The structural and zinc-binding properties of PA4063, one of the periplasmic proteins expressed by Pseudomonas aeruginosa under zinc-deficient conditions, are presented. PA4063 has a noncanonical ferredoxin-like fold. Two zinc-binding sites with micromolar affinity are exposed and are located on the same face of the structure. Two histidine-rich loops, which are disordered in the apoprotein, contribute to zinc coordination in one of the sites. These findings strongly suggest a role for PA4063 in zinc trafficking, possibly acting as a metal chaperone or as a regulator of a transport system.

PA4063 crystallized in two different forms corresponding to space groups P41212 and P65. The asymmetric unit of the hexagonal crystal comprises three protein molecules, but the interactions are so limited that they can be considered as simple packing contacts between monomers as in the case of the tetragonal crystal form. This observation is in line with size-exclusion chromatography, which shows that the protein is monomeric in solution regardless of the presence of zinc. Despite the differences in crystal packing with regard to both lattice and asymmetric unit composition, the conformation of the protein in the two crystal forms is almost identical (Cα r.m.s.d. in the range 0.49–0.74 Å).

>HDDHDHDHAHGSLGKHEHGVAQLNVALDGKTLELELDSPAMNLVGFEHAASTDADKAAVAKARAQLEKPLELFALPVTAGCSVASQELRSPLFGDKAPAHAHKEKAGHEHEHEHEHEHGHADIHAHYQLSCEKPELLKLLTLAEFFKRFPATQKIQVQLIGPDGQKGADLAPASAELKL[3x]> MVSQETIKHVKDLIAENEIFVASKTYCPYSHAAL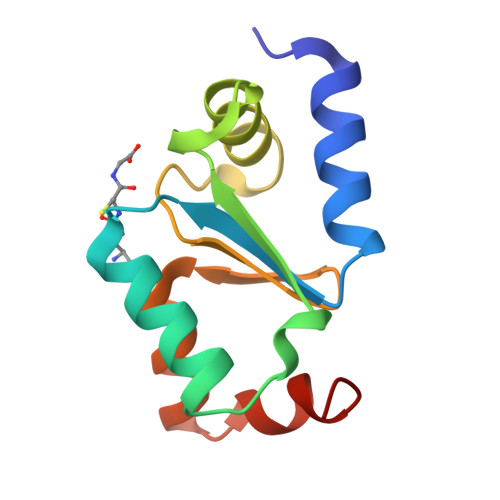NTLFEKLKVPRSKVLVLQLNDMKEGADIQAALYEINGQRTVPNIYINGKHIGGNDDLQELRETGELEELLEPILAN>[2x]MTTLAIDIGGTKLAAALIGADGQIRDRRELPTPASQTPEALRDALSALVSPLQAHAQRVAIASTGIIRDGSLLALNPHNLGGLLHFPLVKTLEQLTNLPTIAINDAQAAAWAEFQALDGDITDMVFITVSTGVGGGVVSGCKLLTGPGGLAGHIGHTLADPHGPVCGCGRTGCVEAIASGRGIAAAAQGELAGADAKTIFTRAGQGDEQAQQLIHRSA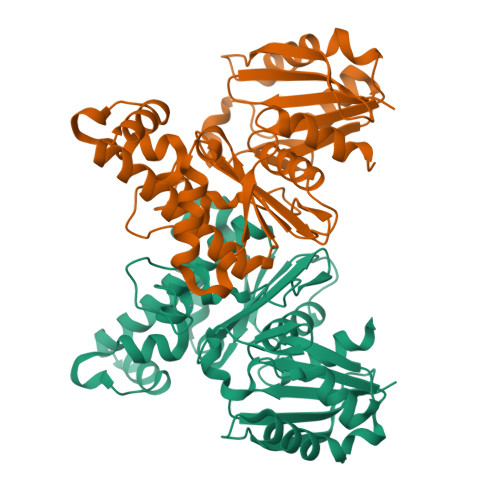RTLARLIADIKATTDCQCVVVGGSVGLAEGYLALVETYLAQEPAAFHVDLLAAHYRHDAGLLGAALLAQGE> FACKTANGTAIPIGGGSANVYVNLAPVVNVGQNLVVDLSTQIFCHNDYPETITDYVTLQRGSAYGGVLSNFSGTVKYSGSSYPFPTTSETPRVVYNSRTDKPWPVALYLTPVSSAGGVAIKAGSLIAVLILRNTNNYNSDDFQFVWNIYANNDVVVPTGGCDVSARDVTVTLPDYPGSVPIPLTVYCAKSQNLGYYLSGTTADAGNSIFTNTASFSPAQGVGVQLTRNGTIIPANNTVSLGAVGTSAVSLGLTANYARTGGQVTAGNVQSIIGVTFV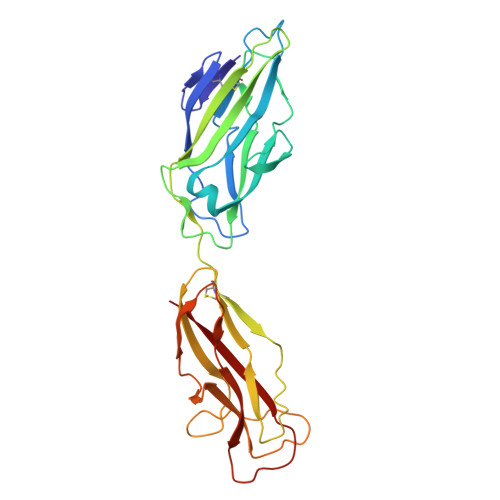YQ> HHHHHHMAKSDVKLLGAWPSPFVMRPRI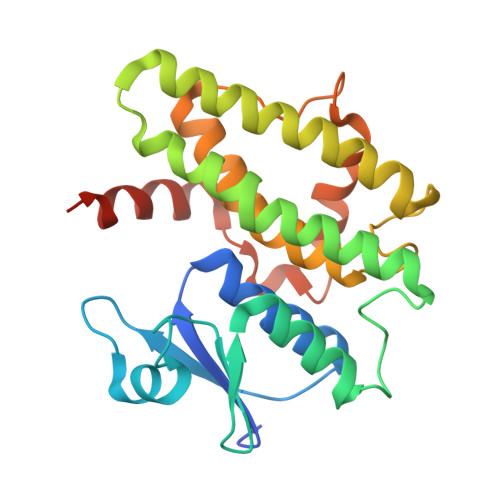ALNIKSVEYEFLEETLGSKSQLLLESNPVHKKTPVLIHGGKPICESLVIVEYIDEVWSPGPAILPSDPYDRALARFWAAYLDEKWFPTMRNIAAAKDEEARKALIDQVGEGLVLLEDAFSKCSKGKGFFGGDQIGYLDIAFGSFLGWLRAIEKMNGVKLMDETRTPGLLKWANSFSSHPAVKDVFPETEKLVEFAKVLAKLKATPPK6-[2-(hydroxymethyl)phenyl]isoquinolin-1(2H)-one 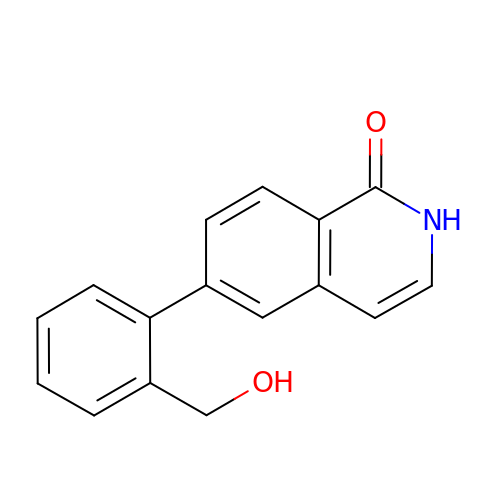| C16 H13 N O2 | UYPQNXCIONEUFC-UHFFFAOYSA-N>[2x]SMTIRFHRNDLPNLDNYQVDAVAIDTETLGLNPH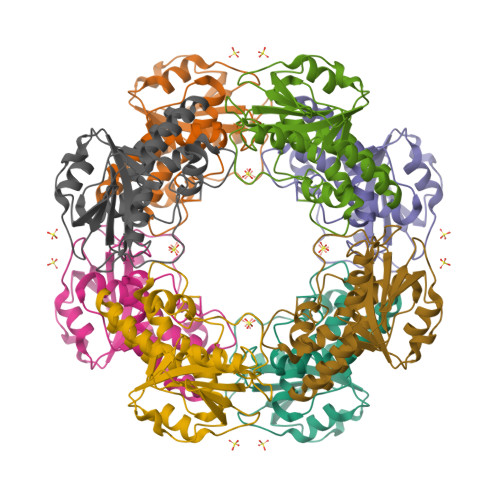RDRLCVVQISPGDGTADVIQIEAGQKKAPNLVKLLKDRSITKIFHFGRFDLAVLAHAFGTMPQPVFCTKIASKLTRTYTDRHGLKEICSELLDVSISKQQQSSDWAAEVLSQAQLEYAASDVLYLHRLKAVLEQRLERDGRTKQAEACFKFLPTRSELDLMGWAESDIFAHS>MQKYVCNVCGYEYDPAEHDNVPFDQLPDDWCCPVCGVSKDQFS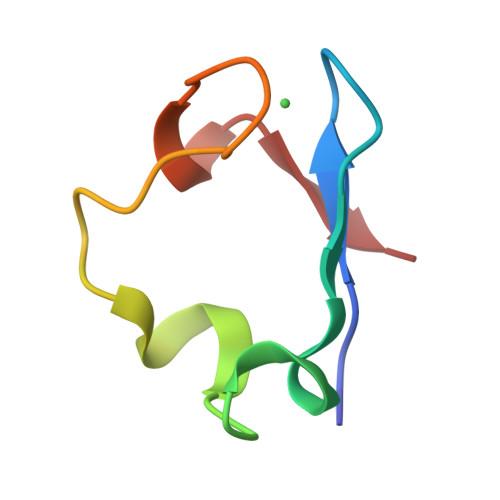PA[2x]>MGSSHHHHHHSSGLVPAGSHSKVFIRSAINRVHQNSAANGGELPRIVFPEGTSTKVLKALATLVEEKICQPILLGYPERVKEKIKALDIPLLNDVSIVHPSSHPKYFSFVEKLYSLRQRKGINLGEAERLMADPNYFAAMMVNQGEADGMVSGSSINYADAVRPILQTIGVYKEGIPAGLNFVLLEDKFLVLADTTVNLNPTAEQCAQIALQAAKIVEYFGIEPRVAMLSYSNFSGAEGTPRKMKKAAEIARSLRPDLMIEGDMQADTAVNPEIMERLFPFSGLKGGANVLVFPNLESSNIAYKLIQQIGKAEVIGPFLTGVRRSANVLQRTTTVDGIVNSVVFTALEAQYIKEVLKSRGKK[12x]

Bacterial hybrid malic enzymes (MaeB grouping, multidomain) catalyse the transformation of malate to pyruvate, and are a major contributor to cellular reducing power and carbon flux. Distinct from other malic enzyme subtypes, the hybrid enzymes are regulated by acetyl-CoA, a molecular indicator of the metabolic state of the cell. The larger ME isoforms (hybrid enzymes) are predicted to be a fusion of two unrelated enzymes; a catalytic N-terminal ME subunit and a C-terminal phosphotransacetylase (PTA) domain. The PTA domain is homologous to PTA enzymes (that interconvert acetyl-CoA and phosphate to CoA and acetyl phosphate), yet they appear to lack critical catalytic residues and thus acts as a sensor instead.

To verify these findings without using mutation, we were inspired by flavoprotein methods used to remove tightly-bound FMN32, and used a moderate Br−/urea wash step to generate ligand-free MaeB. Washed samples of the native MaeBPTA PTA-only construct (hereafter referred to as PTAapo) were crystallised and diffracted to 2.72 Å resolution. PTAapo retains the same D3 symmetry as the acetyl CoA bound form, and, in agreement with our HPLC data, there was a clear lack of ligand electron density. Loss of ligand binding results in locally small changes; however, the use of d2 as a stator and d1 as a flexor means that these small alterations are magnified at the isologous d1:d1 interface. When superimposing the two states via d2, it is apparent that acetyl-CoA attracts the 3′ loop, pulling d1 and d2 closer together.N-ACETYL SEROTONIN | C12 H14 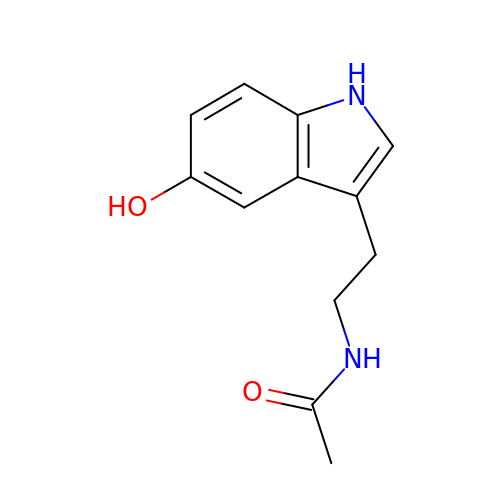N2 O2 | MVAWJSIDNICKHF-UHFFFAOYSA-N> ERSSNNFNYGAYHSLEAIYHEMDNIAADFPDLARRVKIGHSFENRPMYVLKFSTGKGVRRPAVWLNAGIHSREWISQATAIWTARKIVSDYQRDPAITSILEKMDIFLLPVANPDGYVYTQTQNRLWRKTRSRNPGSSCIGADPNRNWNASFAGKGASDNPCSEVYHGPHANSEVEVKSVVDFIQKHGNFKGFIDLHSYSQLLMYPYGYSVKKAPDAEELDKVARLAAKALASVSGTEYQVGPTCTTVYPASGSSIDWAYDNGIKFAFTFELRD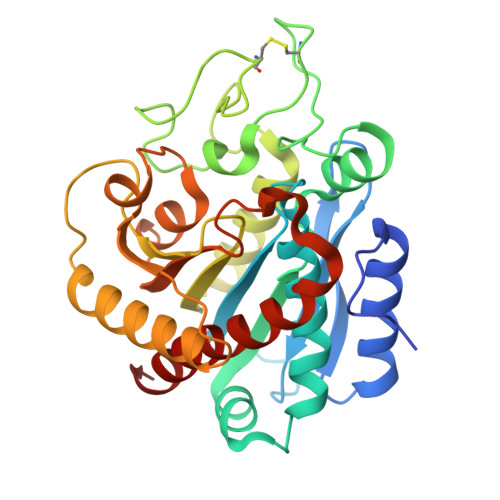TGTYGFLLPANQIIPTAEETWLGLKTIMEHVRDNLY>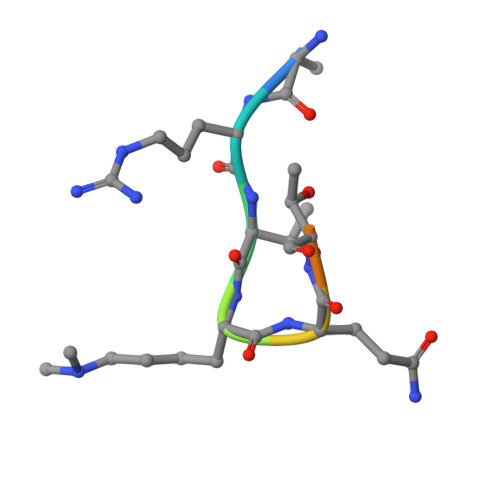 ARTKQTARK> MADNLPSDFDVIVIGTGLPESIIAAACSRSGQRVLHVDSRSYYGGNWASFSFSGLLSWLKEYQENNDVVTENSMWQEQILENEEAIPLSSKDKTIQHVEVFCYASQDLHKDVEEAGALQKNHASVTSAQSAEAAEAAETSCLPTAVEPLSMGSCEIPAEQSQCPGPESSPEVNDAEATGKKENSDAKSSTEEPSENVPKVQDNTETPKKNRITYSQIIKEGRRFNIDLVSKLLYSRGLLIDLLIKSNVSRYAEFKNITRILAFREGTVEQVPCSRADVFNSKQLTMVEKRMLMKFLTFCVEYEEH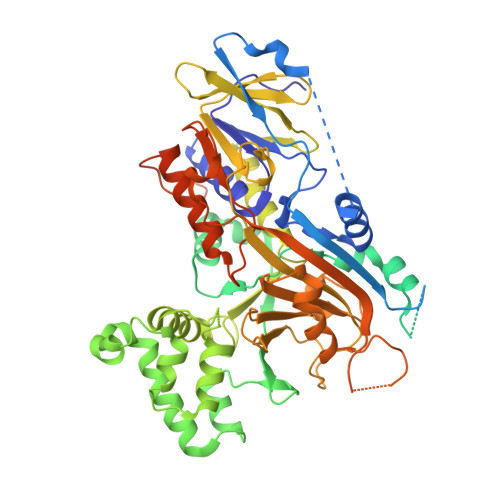PDEYRAYEGTTFSEYLKTQKLTPNLQYFVLHSIAMTSETTSCTVDGLKATKKFLQCLGRYGNTPFLFPLYGQGELPQCFCRMCAVFGGIYCLRHSVQCLVVDKESRKCKAVIDQFGQRIISKHFIIEDSYLSENTCSRVQYRQISRAVLITDGSVLRTDADQQVSILTVPAEEPGSFAVRVIELCSSTMTCMKGTYLVHLTCMSSKTAREDLERVVQKLFTPYTEIEAENEQVEKPRLLWALYFNMRDSSDISRDCYNDLPSNVYVCSGPDSGLGNDNAVKQAETLFQQICPNEDFCPAPPNPEDIVLDGDSSQQEVPESSVTPETNSETPKESTVLGNPEEPSE> ADKELKFLVVDDFSTMRRIVRNLLKELGFNNVEEAEDGVDALNKLQAGGYGFVISDWNMPNMDGLELLKTIRADGAMSALPVLMVTAEAK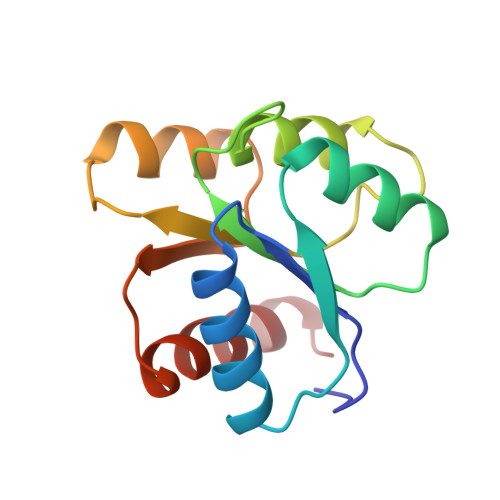KENIIAAAQAGASGYVVKPFTAATLEEKLNKIFEKLGM>[2x]MHHHHHHSRPKLVTWMNNQRVGELTKLANGAHTFKYAPEWLASRYARPLSLSLP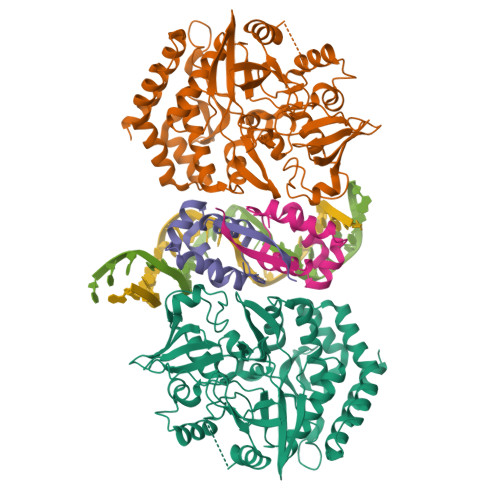LQRGNITSDAVFNFFDNLLPDSPIVRDRIVKRYHAKSRQPFDLLSEIGRDSVGAVTLIPEDETVTHPIMAWEKLTEARLEEVLTAYKADIPLGMIREENDFRISVAGAQEKTALLRIGNDWCIPKGITPTTHIIKLPIGEIRQPNATLDLSQSVDNEYYCLLLAKELGLNVPDAEIIKAGNVRALAVERFDRRWNAERTVLLRLPQEDMCQTFGLPSSVKYESDGGPGIARIMAFLMGSSEALKDRYDFMKFQVFQWLIGATQGHAKNFSVFIQAGGSYRLTPFYDIISAFPVLGGTGIHISDLKLAMGLNASKGKKTAIDKIYPRHFLATAKVLRFPEVQMHEILSDFARMIPAALDNVKTSLPTDFPENVVTAVESNVLRLHGRLSREYGSK;>GSHMMSFQKIYSPTQLANAMKLVRQQNGWTQSELAKKIGIKQATISNFENNPDNTTLTTFFKILQSLELSMTLCDTKNASPESTEQQDLEW[2x]> GAMASKLRLQLDAHASIHENVRRLLQFTTSIMEANEEGIRKDIDSEFLHDFRVAIRRSRSILRLLNGVFDPEKTAWMLAGLRELGKRTNDLRDSDVYLLRREEYTSLLPPSLRPALDPFFSDLEADKRLHHRQFCRYLTGREYSGFMTSLKEFIAEGELPDPETAPLAAEPTGDVAAKTIRKALKKVLVHGRRTGSETSDAELHELRIDCKKLRYLLEFFASLFPPKATAQVLRQMKTLQDNLGTFVDLTVQMEFLQSRLETIPADRGGISEAAAIGGLLTTLYRKREKVREHFHEIFSGFDSNETGELFDELLTGLA

Here, we report that bacterial, archaeal, and eukaryotic conserved histidine α-helical (CHAD) domains are specific polyP-binding modules. All CHAD domains fold into two 4-helix bundles with up-down-up-down topology. Analysis of the surface charge distribution in the different CHAD domains revealed a highly basic central cavity, which is surrounded by two basic surface patches on each side. The basic amino acids contributing to these surface patches are highly conserved among different CHAD proteins.

We next compared the refined structures of the plant CHAD domain to the bacterial CtCHAD and ygiF structures. Notably, helices α4/α5 and α10/α11 are protruding the bundle cores in the RcCHAD and CtCHAD structures, forming a small pore in the center of the domain, which we find to be absent in our ygiF structure. This rationalizes the presence of “long” (∼300 amino acids, e.g., RcCHAD and CtCHAD) and “short” (∼200 amino acids, e.g., ygiF and SsCHAD) CHAD domains. Analytical size-exclusion chromatography experiments indicated that the different CHAD proteins adopt different oligomeric states in solution, with ygiF and SsCHAD behaving as monomers, whereas unliganded CtCHAD form dimers in solution (see the Discussion section). In line with this, size-exclusion chromatography coupled to right-angle light scattering (SEC-RALS) revealed the presence of CtCHAD dimers and tetramers in the absence of polyP. Addition of a long-chain polyP shifted CtCHAD into tetrameric and higher oligomeric states. It is of note that CtCHAD also shows a crystal packing consistent with a dimer or tetramer, which would enable cooperative binding of several CHAD domains to a single polyP chain. The sensograms of CtCHAD and ygiF binding to polyP could only be explained using a heterogeneous analyte model. We speculate that different oligomeric states observed with the CHAD domains used in this study may account for this behavior. However, heparin, which is absent in bacteria and plants, was bound by CtCHAD with binding constants comparable to those determined for polyP.> GSPLLDDDDQVAFSFILDNIVTQKMMAVPDSWPFHHPVNKKFVPDYYKVIVNPMDLETIRK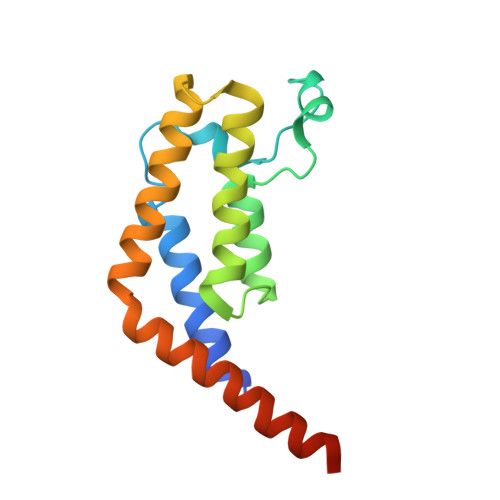NISKHKYQSRESFLDDVNLILANSVKYNGPESQYTKTAQEIVNVCYQTLTEYDEHLTQLEKDICTAKEAALEEAELESLDPMT> SNAMVKIEVAKPINFNRLITSKEAEVVSMRILNQPNSYISLFSLAKDEEITAEAMLGNRYYYCFNGNGEIFIENNKKTISNGDFLEITANHNYSIEARDN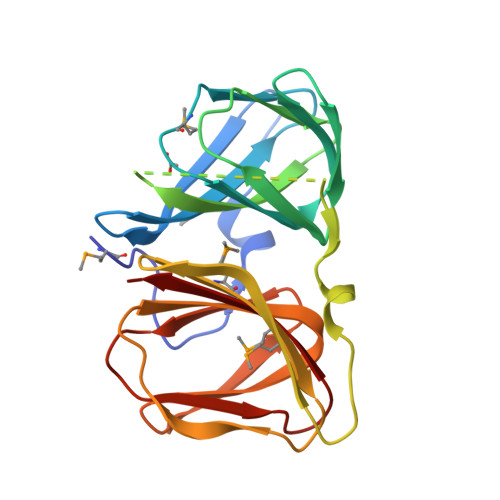LKLIEIGEKIGDGNMENKTLKMLESASAFNLAEVVEYQEGKIVSKNLVAKPNLVMTIMSFWKGESLDPHKAPGDALVTVLDGEGKYYVDGKPFIVKKGESAVLPANIPHAVEAETENFKMLLILVKE> GSMESAQAVAEPLDLVRLSLDEIVYVKLRGDRELNGRLHAY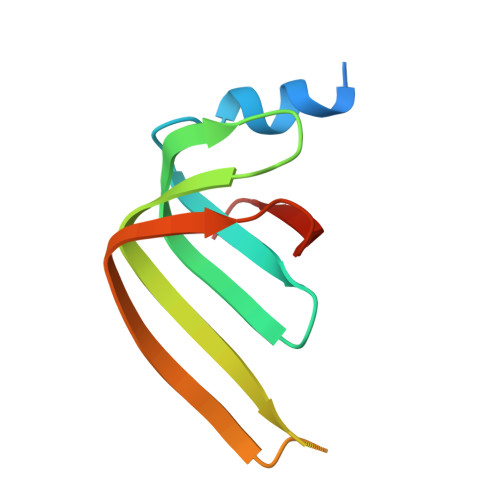DEHLNMVLGDAEEIVTIFDDEETDKDKALKTIRKHYEMLFVRGDSVILIAPPRN>[2x]SLKVNHTKSIGLLATSSEAAYFAEIIEAVEKNCFQKGYTLILGNAWNNLEKQRAYLSMMAQKRVDGLLVMCSEYPEPLLAMLEEYRHIPMVVMDWGEAKADFTDAVIDNAFEGGYMAGRYLIERGHREIGVIPGPLERNTGAGRLAGFMKAM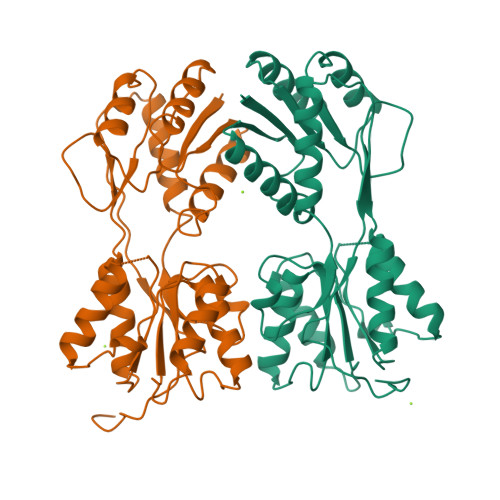EEAMIKVPESWIVQGDFEPESGYRAMQQILSQPHRPTAVFCGGDIMAMGALCAADEMGLRVPQDVSLIGYDNVRNARYFTPALTTIHQPKDSLGETAFNMLLDRIVNKREEPQSIEVHPRLIERRSVADGPFRDYRR>[2x]GMTKEASRPALDLARQAYEAFKARGLNLNMQRGQPADADFDLSNGLLTVLGAEDVRMDGLDLRNYPGGVAGLPSARALFAGYLDVKAENVLVWNNSSLELQGLVLTFALLHGVRGSTGPWLSQTPKMIVT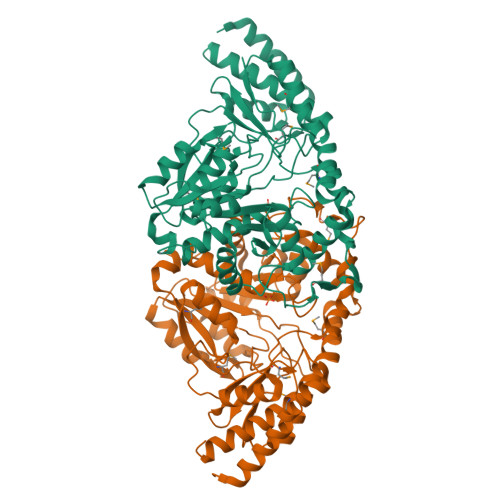VPGYDRHFLLLQTLGFELLTVDMQSDGPDVDAVERLAGTDPSVKGILFVPTYSNPGGETISLEKARRLAGLQAAAPDFTIFADDAYRVHHLVEEDRAEPVNFVVLARDAGYPDRAFVFASTSKITFAGAGLGFVASSEDNIRWLSKYLGAQSIGPNKVEQARHVKFLTEYPGGLEGLMRDHAAIIAPKFRAVDEVLRAELGEGGEYATWTLPKGGYFISLDTAEPVADRVVKLAEAAGVSLTPAGATYPAGQDPHNRNLRLAPTRPPVEEVRTAMQVVAACIRLATEEYRAGH> KDTIALVVSTLNNPFFVSLKDGAQKEADKLGYNLVVLDSQNNPAKELANVQDLTVRGTKILLINPTDSDAVGNAVKMANQANIPVITLDRQATKGEVVSHIASDNVLGGKIAGDYIAKKAGEGAKVIELQGIAGTSAARERGEGFQQAVAAHKFNVLASQPADFDRIKGLNVMQNLLTAHP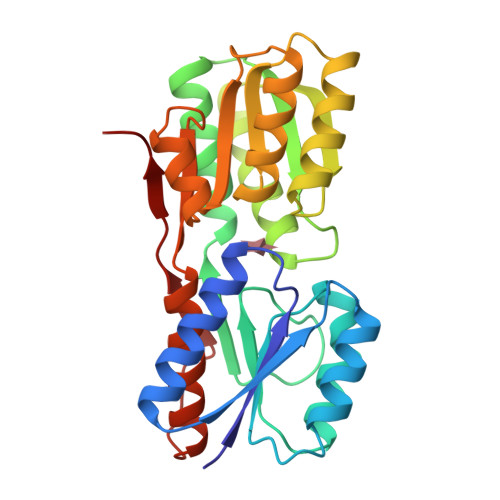DVQAVFAQNDEMALGALRALQTAGKSDVMVVGFDGTPDGEKAVNDGKLAATIAQLPDQIGAKGVETADKVLKGEKVQAKYPVDLKLVVKQ>[3x]MIDQKEKELIKESWKRIEPNKNEIGLLFYANLFKEEPTVSVLFQNPISSQSRKLMQVLGILVQGIDNLEGLIPTLQDLGRRHKQYGVVDSHYPLVGDCLLKSIQEYLGQG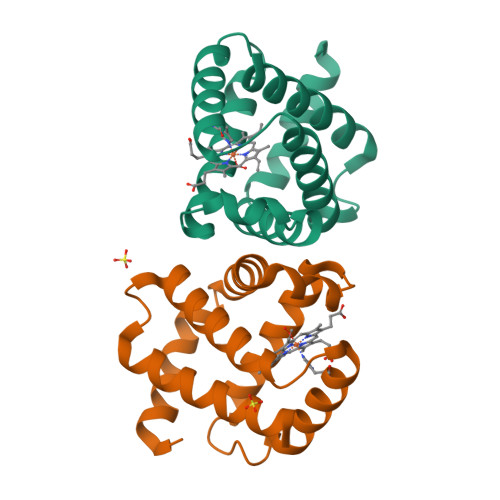FTEEAKAAWTKVYGIAAQVMTAEHHHHHH> HHAADYVLYKDATKPVEDRVADLLGRMTLAEKIGQMTQIERLVATPDVLRDNFIGSLLSGGGSVPRKGATAKEWQDMVDGFQKACMSTRLGIPMIYGIDAVHGQNNVYGATIFPHNVGLGATRDPYLVKRIGEATALEVRATGIQYAFAPCIAVCRDPRWGRCYESYSEDRRIVQSMTELIPGLQGDVPKDFTSGMPFVAGKNKVAACAKHFVGDGGTVDGINENNTIINREGLMNIHMPAYKNAMDKGVSTVMISYSSWNGVKMHANQDLVTGYLKDTLKFKGFVISDWEGIDRITTPAGSDYSYSVKASILAGLDMIMVPNKYQQFISILTGHVNGGVIPMSRIDDAVTRILRVKFTMGLFENPYADPAMAEQLGKQEHRDLAREAARKSLVLLKNGKTSTDAPLLPLPKKAPKILVAGSHADNLGYQCGGWTIEFQGDTGRTTVGTTILEAVKAAVDPSTVVVFAENPDAEFVKSGGFSYAIVAVGEHPYTETKGDNLNLTIPEPGLSTVQAVCGGVRCATVLISGRPVVVQPLLAASDALVAAWLPGSEGQGVTDALFGDFGFTGRLPRTWFKSVDQLPMNVGDAHYDPLFRLGYGLTTNATKKY

In the barley β-d-glucan glucohydrolase, a glycoside hydrolase family 3 (GH3) enzyme, the Trp286/Trp434 clamp ensures β-d-glucosides binding, which is fundamental for substrate hydrolysis during plant growth and development. HvExoI folds into a two-domain structure consisting of an (α/β)8 barrel (domain 1) and an (α/β)6 sandwich (domain 2) with a 13 Å-deep active site pocket embracing the subsites −1 and +1, positioned at the interface between the two domains. HvExoI catalyses the hydrolytic removal of nonreducing glucose (Glc) moiety from a broad spectrum of poly- and oligomeric β-d-glucosides. The crucial role of substrate binding in HvExoI implies a pair of the aromatic Trp286 and Trp434 residues that form a clamp at the +1 subsite, which is positioned next to a pocket-shaped site at the −1 subsite, housing the Asp285 and Glu491 catalysts.

G6SG-OMe bound tightly to native and WT recombinant HvExoI with the respective Ki values of 0.1 ×10−3 M and 0.2 ×10−3 M, hinting that this thio-analogue should be observed in the active sites of WT and mutants. This is what we indeed observed in WT, and the W286A, W286Y, W286F, W434A, W434F, W434H, and W434Y mutants, where well-defined electron density maps of G6SG-OMe and tight H-bond networks that were formed through eight to ten residues (Asp95, Lys206, His207, Arg158, Tyr253, Asp285, Arg291, Glu491, Trp286, and Trp434). As expected, the (1,3)- and (1,4)-linked thio-inhibitors were less potent with tested mutants, while the most effective thio-inhibitor was G6SG-OMe, except that it did not bind to W434A, and compared to WT, it showed 8- and 6-fold higher Ki constant values with W434H and W434F, respectively. We noted that the quality of the G6SG-OMe electron density map slightly declined in W286Y but that these maps were well-formed in W286A and W286F, suggesting that in the W286Y mutant the process of ligand-binding in (or near) the active site may have been perturbed. These findings reinforce the conclusion that G6SG-OMe binds in HvExoI regardless of mutations (particularly into aromatic residues) of Trp286 or Trp434.> LSSPQTRYIPDEADFLLGMATVNNCVSYRNPAEGTWYIQSLCQSLRERCPRGDDILTILTEVNYEVSNKDDKKNMGKQMPQPTFTLRKKLVF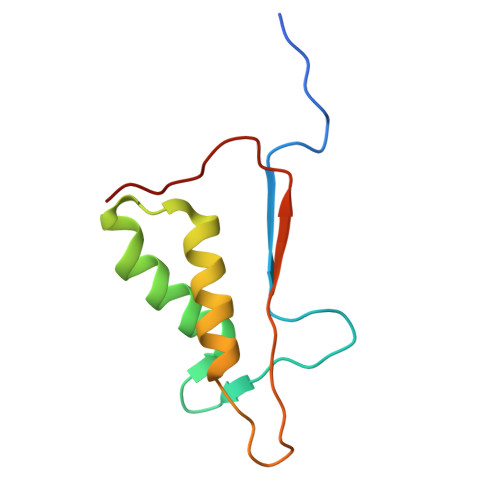PSD> GSHMAVTGSQTALLLRAFEKDRFPGIAAREELARETGLPESRI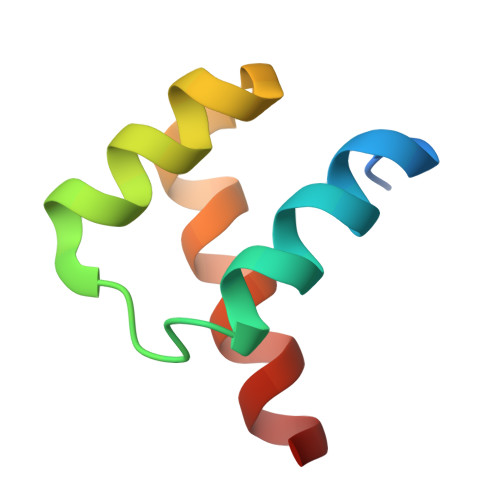QIWFQNRRARHP> MGKITLYEDRGFQGRHYECSSDHTNLQPYLSRCNSASVDSGCWMLYEQPNYSGLQYFLRRGDYADHQQWMGLSDSVRSCRLIPHSGSHRIRLYEREDYRGQMIEFTEDCSCLQDRFRF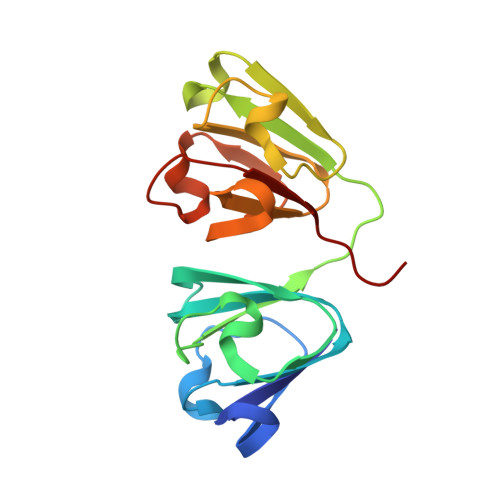NEIHSLNVLEGSWVLYELSNYRGRQYLLMPGDYRRYQDWGATNARVGSLRRVIDFS>[2x]MCLEDSDAGASNEYDSSPAAWNKEDFPWSGKVKDILQNVFKLEKFRPLQLETINVTMAGKEVFLVMPTGGGKSLCYQLPALCSDGFTLVICPLISLMEDQLMVLKQLGISATMLNASSSKEHVKWVHAEMVNKNSELKLIYVTPEKIAKSKMFMSRLEKAYEARRFTRIAVDEVHCCSQWGHDFRPDYKALGILKRQFPNASLIGLTATATNHVLTDAQKILCIEKCFTFTASFNRPNLYYEVRQKPSNTEDFIEDIVKLINGRYKGQSGIIYCFSQKDSEQVTVSLQNLGIHAGAYH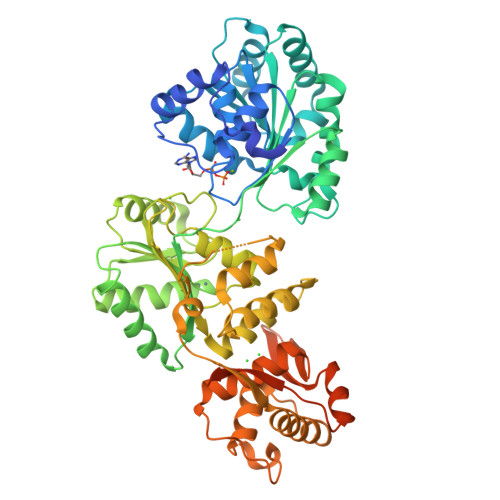ANLEPEDKTTVHRKWSANEIQVVVATVAFGMGIDKPDVRFVIHHSMSKSMENYYQESGRAGRDDMKADCILYYGFGDIFRISSMVVMENVGQQKLYEMVSYCQNISKCRRVLMAQHFDEVWNSEACNKMCDNCCKDSAFERKNITEYCRDLIKILKQAEELNEKLTPLKLIDSWMGKGAAKLRVAGVVAPTLPREDLEKIIAHFLIQQYLKEDYSFTAYATISYLKIGPKANLLNNEAHAITMQVTKSTQNSFRAESSQTCHSEQGDKKMEAENLYFQSHHHHHHDYKDDDDK Microtubule (MT) nucleation is regulated by the γ-tubulin ring complex (γTuRC), conserved from yeast to humans. In budding yeast, homologues of the grip-containing proteins (GCPs) GCP2 and GCP3 (Spc97p and Spc98p) and two copies of γ–tubulin (Tub4p) form a 300 kDa complex (γTuSC). Spc110p, a distant pericentrin homologue, recruits this complex to the nuclear face of the spindle pole body (SPB), while Spc72p recruits it to the cytoplasmic face. In yeast, the CM1 motif is required for seven identical γTuSCs to helically assemble into a γTuRC at the SPB.

To better resolve fundamental questions about the molecular basis for γTuRC assembly and activation, we determined the cryo-EM structure of unassembled γTuSC, without Spc110p or filament formation, from images of frozen-hydrated single particles. At the concentration of ~1 µM used in data collection, micrographs and 2D classes show a mixture of γTuSC monomers and dimers, with a small number of larger oligomers. We were able to obtain a structure of the γTuSC monomer at ~3.7 Å, and of a γTuSC dimer at ~4.5 Å resolution (Figure 5—figure supplements 2 and 3). As initially observed in negative stain EM, our new cryo-EM structures of monomeric and dimeric γTuSCs show that Spc97p and Spc98p intrinsically adopt an open conformation at the intra-γTuSC interface such that the attached γ-tubulins fail to make MT-like lateral contacts. In order to assess the changes that occur during assembly of monomeric γTuSCs into the γTuRC and the subsequent closure, we aligned the N-terminal two helical bundles of Spc97p and Spc98p (residues Spc97p52-276 and Spc98p178-342). During the transition from monomer to assembled open state (as seen in γTuRCWT), the γ-tubulins move in the same overall direction, approximately orthogonal to the plane of the Spc97p/Spc98p contact interface. The center of mass of the γ-tubulins shifts ~13.8 Å and ~15.6 Å when bound to Spc97p and Spc98p, respectively, as a result of twisting the helical bundles in Spc97p and Spc98p. The large conformational change in Spc98p that occurs to create these contacts in the γTuSC dimer is a major contributor to the even larger-scale changes during γTuRC assembly and activation.

>[2x]MGGEIITLQAGQCGNHVGKFLWSQLAKEHAIGTDGLSQLPDSSTERDDDTKPFFRENSRNKFTPRAIMMDSEPSVIADVENTFRGFFDPRNTWVASDGASAGNSWANGYDIGTRNQDDILNKIDKEIDSTDNFEGFQLLHSVAGGTGSGLGSNLLEALCDRYPKKILTTYSVFPARSSEVVVQSYNTILALRRLIEDSDATVVFDNASLLNISGKVFRNPNIDLQHTNQLISTIISSVTNSIRFPSYMYSSMSSIYSTLIPSPELHFLSPSFTPFTSDYIHDDIAHKGHSSYDVMLDLLDPSNSLVSTAMNNPTYFNVYNTIIGNVEPRQISRAMTKLQQRIKFPSWSSSAMHVNIGRRSPYLPLQPNENEVSGMMLSNMSTVVNVFENACNTFDKVFAKGAFLNNYNVGDLFQSMQNVQDEFAESREVVQSLMEDYVAAEQDSYLDDVLVDDENMVGELEEDLDADGDHKLV;> MELEPTLFGIIEALAPQLLSQSHLQTFVSDVVNLLRSSTKSATQLGPLIDFYKLQSLDSPETTIMWHKIEKFLDALFGIQNTDDMVKYLSVFQSLLPSNYRAKIVQKSSGLNMENLANHEHLLSPVRAPSIYTEASFENMDRFSERRSMVSSPNRYVPSSTYSSVTLRQLSNPYYVNTIPEEDILKYVSYTLLATTSALFPFDHEQIQIPSKIPNFESGLLHLIFEAGLLYQSLGYKVEKFRMLNISPMKKALIIEISEELQNYTAFVNNLVSSGTVVSLKSLYREIYENIIRLRIYCRFTEHLEELSGDTFLIELNIFKSHGDLTIRKIATNLFNSMISLYYEYLMNWLTKGLLRATYGEFFIAENTDTNGTDDDFIYHIPIEFNQERVPAFIPKELAYKIFMIGKSYIFLEKYCKEVQWTNEFSKKYHVLYQSNSYRGISTNFFEIINDQYSEIVNHTNQILNQKFHYRDVVFALKNILLMGKSDFMDALIEKANDILATPSDSLPNYKLTRVLQEAVQLSSLRHLMNSPRNSSVINGLDARVLDLGHGSVGWDVFTLDYILYPPLSLVLNVNRPFGRKEYLRIFNFLWRFKKNNYFYQKEMLKSNDIIRSFKKIRGYNPLIRDIINKLSRISILRTQFQQFNSKMESYYLNCIIEENFKEMTRKLQRTENKSQNQFDLIRLNNGTIELNGILTPKAEVLTKSSSSKPQKHAIEKTLNIDELESVHNTFLTNILSHKLFATNTSEISVGDYSGQPYPTSLVLLLNSVYEFVKVYCNLNDIGYEIFIKMNLNDHEASNGLLGKFNTNLKEIVSQYKNFKDRLYIFRADLKNDGDEELFLLSKSLR;> MEIKEVDDRAELLRYTNNIPLLGKLVNHQPLWSTNPKLKSFSLEKISAPDQRRVQEALVVKDLLNVLIGLEGTYIRYFNDYEPSDPETPIEFKIAKKMDPSFKTFSRRIVRYGKQYMILTRAYEKWSDTSFGMVLQRFAYEIRRFLEDVYLKTLVERLERDFNKVPNFSIRELEQIINETEVNKQMELLYNIYEEIFREIEERRTNQSSQEDFNNFMDSMKNESSLHLRLMVAFDTTVYPVPKGGAILKIFQQKILENLGDRSSVMFLKKLLNNISQDYCTMLYEWLTQGILNDPYQEFMTYDDLEGKTDNIFDTRDRAWDTQYFIRKDVLLRDCDSEEDKNLLFKMLRTGILLKVVRASLQIPTIPSNSSDITIQEINDFADLMEGSNLELYVDKCYSRANEIFLKLFFQGYDLINVLKHLQQIFLGYQSGHNVLKFLTKNMGELTKHYRNDNNANYDKLLQNFELERQSENPNNLMRQLLMIQFDTETLPQVLSHYLQIYPEVPENNSANDDSDPLMHANNFKNMNAILFDELSKERTGAYHGSNLELYTPKSAIYHLKFDINIPYPLNIIISRTCMIKYQIILRYQLVLQYHSRLLDETWMDLNKTPSWKYRGYSHTVKRRIVRATRVLHAKMNHFIKTIMEYFNQNVIDKEVYSLEKCYRNPTLAVAIQNELEGGLTNIMTNRCLSDLIPLQLQIFDIVYKFCKFIKSMRAKLCQLDPVLYEKHKSGMMKTLNEGYRTNNGGQEDVGYQEDAALELIQKLIEYISNASSIFRKCLINFTQELSTEKFDFYDSSSVDAAGIERVLYSIVPPRSASASSQR> MGVTCVSQMPVAEGKSVQQTVELLTRKLEMLGAEKQGTFCVDCETYHTAASTLGSQGQTGKLMYVMHNSEYPLSCFALFENGPCLIADTNFDVLMVKLKGFFQSAKASKIETRGTRYQYCDFLVKVGTVTMGPSARGI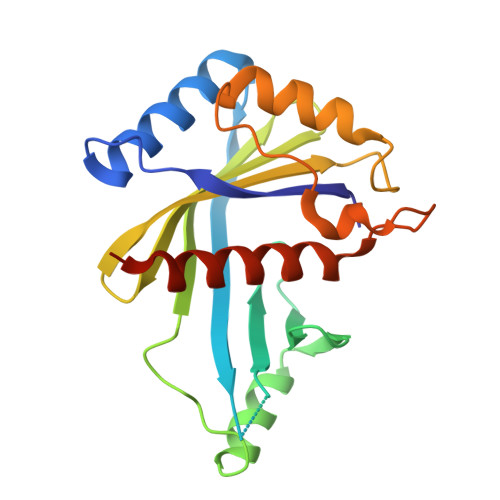SVEVEYGPCVVASDCWSLLLEFLQSFLGSHTPGAPAVFGNRHDAVYGPADTMVQYMELFNKIRKQQQVPVAGIR4-{4-[(3R)-3-methylmorpholin-4-yl]-6-[1-(methylsulfonyl)cyclopropyl]pyrimidin-2-yl}-1H-indole 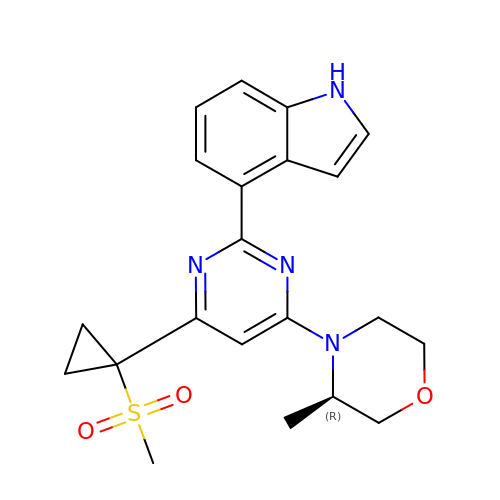| C21 H24 N4 O3 S | SCGCBAAYLFTIJU-CQSZACIVSA-N>[2x]MVSEMLEEIKRTIMQRLPERVQVAKVEFEGPEVVIYTKNPEIITENGNLIRDIAKDIRKRIIIRSDRSVLMDPEKAIRKIHEIVPEEAKITNISFDDVTCEVIIEARKPGLVIGKYGSTSREIVKNTGWAPKILRTPPISSEIIERIRRTLRKNSKERKKILQQLGNRIHQKPKYDNDWARLTAMGGFREVGRSCLYLQTPNSRVLLDCGVNVAGGDDKNSYPYLNVPEFTLDSLDAVIITHAHLDHSGFLPYLYHYGYDGPVYCTAPTRDLMTLLQLDHIDIAHREDEPLPFNVKHVKKSVKHTITLDYGEVTDIAPDIRLTLHNAGHILGSAMAHLHIGDGQHNMVYTGDFKYEQSRLLEAAANRFPRIETLVMESTYGGHEDVQPSRNRAEKELVKTIYSTLRRGGKILIPVFAVGRAQELMIVLEEYIRTGIIDEVPVYIDGMIWEANAIHTARPEYLSKDLRDQIFHMG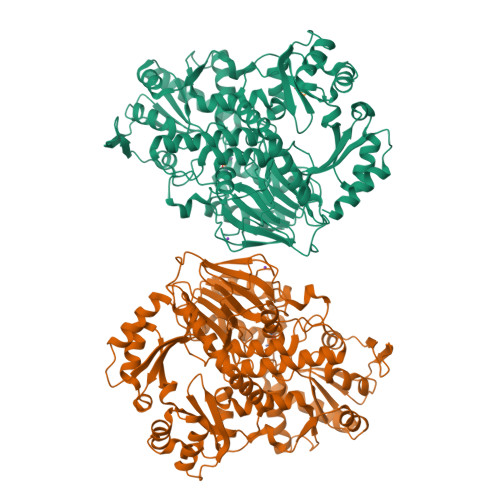HNPFISDIFHKVNGMDERREIVEGEPSIILSTSGMLTGGNSLEYFKWLCEDPDNSLVFVGYQAEGSLGRRIQKGWKEIPLKDEDDKMRVYNVRMNIKTIEGFSGHSDRRQLMEYVKRISPKPEKILLCHGDNYKTLDLASSIYRTYRIETKTPLNLETVRIQ>PKWQAVRAEYQRQRDPLHQFASQQNPEAQLQALQDKIRANPQNSEQWALLGEYYLWQNDYSNSLLAYRQALQLRGENAELYAALATVLYYQASQHMTAQTRAMIDKALALDSNEITALMLLASDAFMQANYAQAIELWQK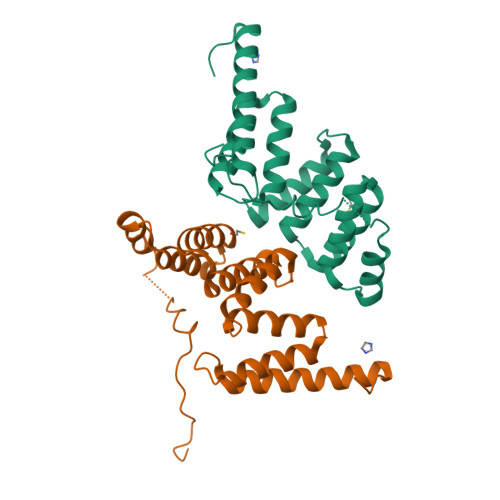VMDLNSPRINRTQLVESINMAKLLQRRSDLEHHHHHH[2x]> MGHHHHHHGQQDVHGPFQGQRQNEFDLMFVKEIFKNHNSNVVLSPFSVKILLTLIYEASDTSFGNAVSNTKRELSSVIQNDNIDHTRSYYKQLLESAQQDNKDYDLNIATNFFVDDFIEVINKYQQIANTHYHAMLEKVSYSNPTQTAATINNWVSEHTNGRLREIVTPDSLEGAVITLVNVIYFKGLWTYPFPEVANNVKPFYGTRGKPTNAQYMEQNGQFYYDNSADLGAQILRLPYRGNKLAMYFILPNPDNT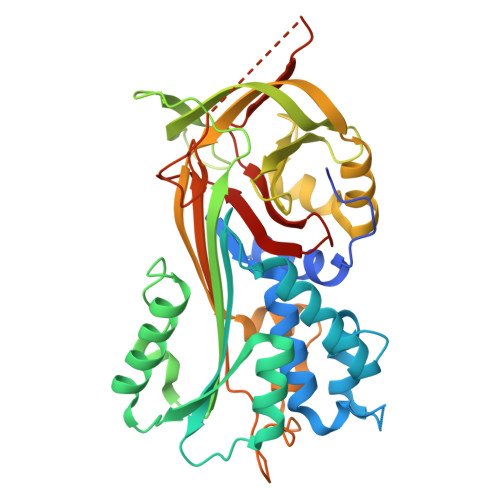VNQVLDRINSASLHQALWYMEENEVNVTLPKFKFDFSEQLNEPLQQVGIREIFSQNASLPLLARGRGARDEVRVSRIFQKAGITINELGSEAYAATEIQLVNKFGGDGVQIFNANRPFIFFIEDETLGTMLFAGKIENPVF(6~{E},10~{E},14~{E},18~{E},22~{E},26~{E},30~{R})-2,6,10,14,18,22,26,30-octamethyldotriaconta-2,6,10,14,18,22,26-heptaene 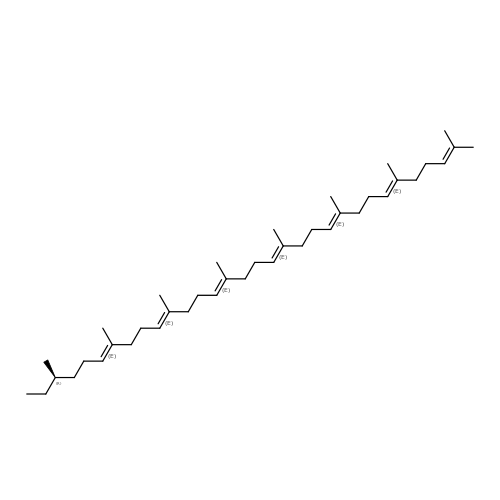| C40 H68 | NNAMSNGZQLVMQY-GAPQENEMSA-N Here, we report two crystal structures of this novel protein family, a circularly permuted imelysin (with the GxHxxE motif) from Bacteroides ovatus (PIBO) and an imelysin-like protein (with a variant GxxxxE motif) from Psychrobacter arcticus 273-4 (IPPA). The PIBO monomer is a V-shaped, all helical structure consisting of two domains, D1 (residues 33–90 and 244–384) and D2 (residues 91–243), with molecular dimensions of 73 Å×55 Å×42 Å. The functional site of PIBO is likely located at the domain interface and supported by the clustering of conserved residues, including the buried GxHxxE motif. As a result, our structural evidence clearly argues against PIBO being a metallopeptidase.

The asu of the final model contains one monomer (A, residues 30–384), two chloride ions, two glycerol molecules, and 533 water molecules. The second PIBO structure at higher resolution contains significantly more residues that display multiple conformations (57 for one monomer) than in crystal form 1 (45 for two monomers). In crystal form 2, a glycerol is found in place of the magnesium. The αO-αR insert (defined as the region between αO and αR) of PIBO adopts different conformations in the two crystal forms. However, helix αQ is unwound before residue 361 in crystal form 2, where the peptide changes its direction towards helix αA. These observed conformational changes are likely influenced by differences in crystal packing and environment. The overall conformation of the αD-αF insert in IPPA is structurally more similar to that of crystal form 2 of PIBO. The middle portion of helix αI (residues 215–231) in the second crystal of PIBO displays discrete structural heterogeneity and a helical shift. The two conformers differ by a main-chain shift, resulting in Cα displacements that vary between 0.6 Å and 1.5 Å. Thus, it appears that this region fluctuates between different sub-states, with its conformation affected by crystal packing or other external factors.

> GSDDDNPTVDPANIDYTPENASSWHNYMRNVAALLKTDATNLYNAWNSSYKGGESYASLFKAHSGSPYASALSCVEEIVDKCAEIANEVGTAKIGDPYNLYKAGNTEEALYAVESWYSWHSRDDYTNNIYSIRNAYYGSLDGNINANSLSTVIAGANSSLDTKIKNAIQKAAKAIQDIPQPFRNHIPSNETVAAMDACAELESILKNDLKSYIANNSNNINTDAVLNPVVTQYVDAVVVPTYKSLKEKNDALYNAVIVLADNPSNSAFETACDAWITAREPWEKSEAFLFGPVDEMGLDPNMDSWPLDQNAIVQILNSQSWSDLEWSEGDDEAAVESAQNVRGFHTLEFLLYKNGEPRKVQ Hydroxynitrile lyase from Hevea brasiliensis (HbHNL) and the esterase SABP2 from Nicotiana tabacum share the α/β-hydrolase fold, a Ser–His–Asp catalytic triad and 44% sequence identity, yet catalyze different reactions. To investigate how regions beyond the active site influence catalytic efficiency and active-site geometry, we engineered HbHNL variants with increasing numbers of substitutions to match SABP2. Variant HNL16 has all amino acids within 6.5 Å of the active site identical to SABP2, HNL40 those within 10 Å and HNL71 those within 14 Å. HNL16 exhibited poor esterase activity, whereas both HNL40 and HNL71 showed efficient esterase catalysis, demonstrating that residues beyond the immediate active site are critical for functional conversion.

Variant HNL71 contains 31 additional substitutions beyond those in HNL40, giving a total of 71, which corresponds to removing approximately one half (49%) of the differences between the proteins. These 31 additional substitutions increase the sequence identity to SABP2 to 71% for HNL71 and expand the region of identical protein sequence with SABP2 to 14 Å from salicylic acid bound in the active site of SABP2. The 31 additional substitutions in HNL71 further increase the kcat value fourfold to 310 min−1, making HNL71 a 2.4-fold better esterase than SABP2. Although the sequence of HNL71 is closer to that of HbHNL (72% sequence identity) by ten amino acids than to SABP2 (68% sequence identity), it shows no significant hydroxynitrile lyase activity and instead is a 2.4-fold better esterase than SABP2. The χ1 angles at histidine, serine and OX2 are within 7° of those in SABP2. Thus, the 71 changes introduced to create HNL71 create nearly, but not completely, identical catalytic atom positions. In HNL71, the data also lacked sufficient electron density to define nine residues in two surface regions: a two-residue segment Gly142-Lys143 in the cap domain and a seven-residue segment Met182-Glu183-Ile184-Leu185-Ala186-Lys187-Arg188 in the catalytic domain. During refinement of HNL71, the Fo − Fc (red/green) electron-density map revealed a notable density adjacent to the sulfur of Cys163 in both chains A and B. Placing an O atom into this density decreased the Rwork and Rfree values. This addition of an O atom suggests that Cys163 has been oxidized to a sulfenic acid in HNL71. The oxidation seen in HNL71 may be due to oxidative conditions encountered by the HNL71 crystal.

>[2x]MAFAHFVLVHGACHGGWSWHKLKPLLEALGHKVTALDLAASGVDPRQIEELGTLDEYTEPLLTFLEALPPGEKVILVGHSLGGMNLGIAADKYCEKIAAAVFLAAFMPDTEHCSSFVLEQYNERTPAENWLDTQFLTYTKDGKEITSMFFGPKFLAHKLYQLCGPEDLELASMLVRPSSLMMEILAKRPFFTKEGYGSIKKIYIVCTEDKGIPEEFQRWQIENYKPDKVYKVEGADHMAMLCKTKELAEILQEVADTYNAAALEHHHHHH> GALSPGGTKQKYKEVVDIEAQRRLNDLAREARIRRAQQAVLRKELIATSTNVIKSEISLRILASECHLTLNGIVEAEAQYKMGGLPKSRLPKIKHPMIVTKWVDYSNKHGFSYQLSTEDIGVLFNNGTTVLRLADAEEFWYISYDDREGWVASHYLLSEKPRELSRHLEVVDFFAKYMKANLSRVSTFGREEYHKDDVFLRRYTRYKPFVMFELSDGTFQFNFKDHHKMAISDGGKLVTYISPSHESTTYPLVEVLKYGEIPGYPESNFREKLTLIKEGLKQKSTIVTVD

Like Plks, Cdc5 contains a Ser/Thr kinase domain followed by a polo-box domain that mediates substrate recognition and sub-cellular localization. The polo-box domain is made up of two polo boxes that together define the p(S/T)-binding pocket. Cdc5 promotes the release of Cdc14 from the nucleolus and regulates the mitotic exit network (MEN)9,16–18 as well as cytokinesis. Here we demonstrate that the polo-box domain of Cdc5 uses distinct surfaces to bind phosphorylated and non-phosphorylated substrates.

We determined the crystal structure of the polo-box domain of Cdc5 using a fragment of Cdc5 that included residues 418–705. Similar to other previously determined structures of Plk1, the extension preceding the polo-box domain (residues 418–459) was disordered in the structure, while residues Leu460-Asp705 adopted the characteristic polo-box domain fold with the first polo-box defined by the β1-β2-β3-β4-β5-β6-α2 structure elements, and the second by the β7-β8-β9-β10-β11-β12-α3-α4 structure elements. The loop connecting the two polo boxes (Ala594-Ser601) was disordered in this structure. The distance between the last ordered residue from the first polo-box (Lys593) and the first ordered residue in the second polo-box (Thr602), as well the conformation of residues Thr602-Asp611 folding back towards β5-β6 rather than reaching across the first polo-box towards α2, suggested that the loop may had been proteolytically cleaved during crystallization. The side chains of Glu553, His569 and His609, as well as that of His524 from a symmetry related molecule, coordinate a zinc metal ion from the crystallization solution. This metal ion further stabilizes the conformation of the ordered portion of the loop and places the phenyl group of Phe603 inside an exposed hydrophobic pocket delimited by Leu546, Trp555, Ile557 and Ala567.>[2x]SMPPHGELQYLGQIQHILRCGVRKDDRTGTGTLSVFGMQARYSLRDEFPLLT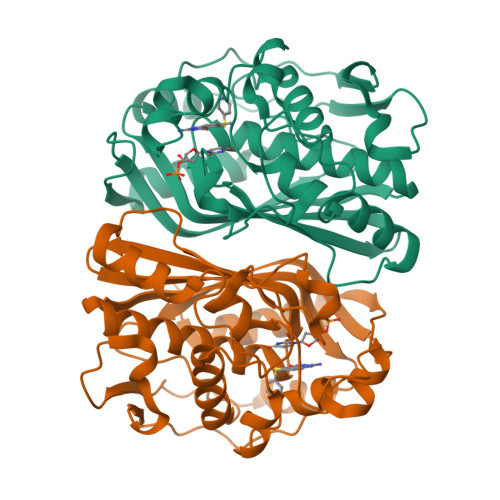TKRVFWKGVLEELLWFIKGSTNAKELSSKGVKIWDANGSRDFLDSLGFSTREEGDLGPVYGFQWRHFGAEYRDMESDYSGQGVDQLQRVIDTIKTNPDDRRIIMCAWNPRDLPLMALPPCHALCQFYVVNSELSCQLYQRSGDMGLGVPFNIASYALLTYMIAHITGLKPGDFIHTLGDAHIYLNHIEPLKIQLQREPRPFPKLRILRKVEKIDDFKAEDFQIEGYNPHPTIKMEMAV>MGHHHHHHHHHHSSGHIEGRHMSRFAADPHWLIYLPPTMSPCETSKKEGMLEHPIEAFEYFRTRGVGKVVCGQKHMGSRAVVIVCKDSQVAEKRFGVLDGTAGICYTRTGRHFFDDMQLEAELIDRVRKVLDKSGFWGDFNTDWVCLDCELMPWSAKAQKLLEEQYSAVGISGRVVLDEAVKLLKQASLNKTVSFDVSRQTSGKNADINELLQR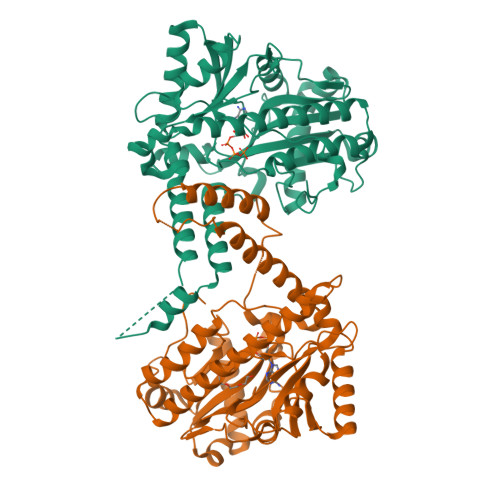FTERSEMMQKYVEAYRKYCWPVNSIDDLKLAPFHILATEGKVHSDKNHIWHMDTIAKYCTQDDSLIMATNHILVDVTDAESVDKGIKWWEDLTASGGEGMVVKPYDFIVKNGRELLQPAVKCRGREYLRIIYGPEYTMDENIERLRNRAVGKKRSLALREFSLGMEALERFVRNEPLYRVHECVFGVLALESEPVDPRL[2x]> STVTNEFCADHPFIYVIRHVDGKIL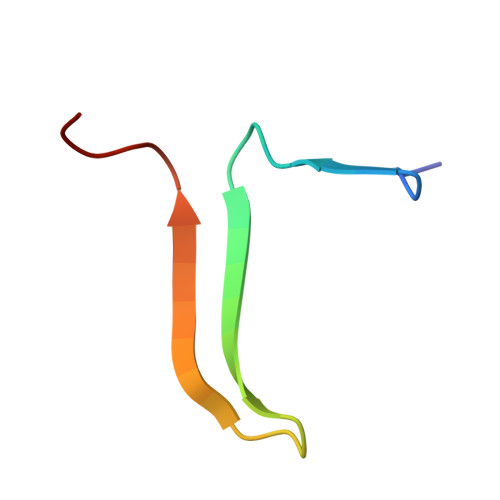FVGRYCSPTTN>HHHHHHSSGLVPRGSHMSFVVIIPARYASTRLPGKPLVDINGKPMIVHVLERARESGAERIIVATDHEDVARAVEAAGGE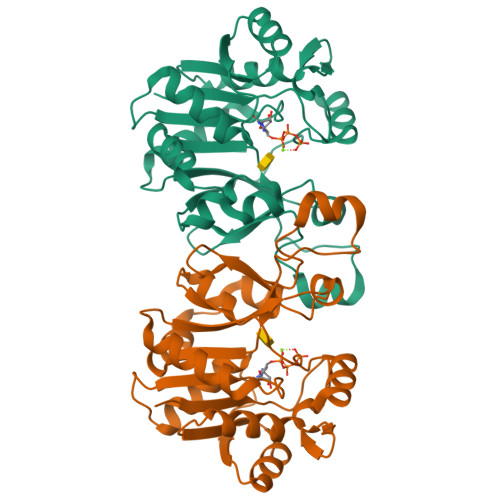VCMTRADHQSGTERLAEVVEKCAFSDDTVIVNVQGDEPMIPATIIRQVADNLAQRQVGMATLAVPIHNAEEAFNPNAVKVVLDAEGYALYFSRATIPWDRDRFAEGLETVGDNFLRHLGIYGYRAGFIRRYVNWQPSPLEHIEMLEQLRVLWYGEKIHVAVAQEVPGTGVDTPEDLERVRAEMR[4x]>[2x]MNMTELKGALIGCGFFAVNQMHAWKDV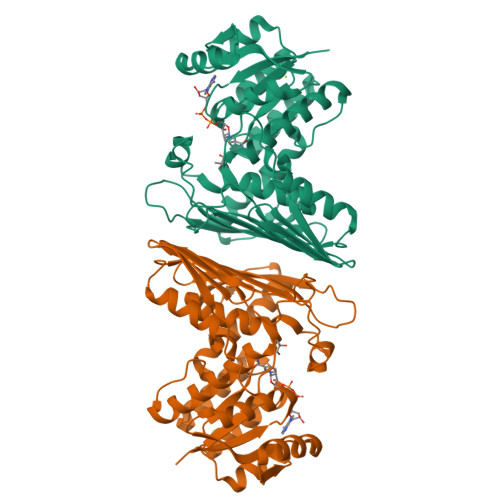KGAGIAAICDRDPKRLKLVGDQFGIERRYGDAAALFADGGFDFVDIATTVQSHRALVEMAAAHKVPAICQKPFAKSLSDAKAMVRTCENADIPLMVHENFRWQTPIQAVKAVLESGAIGEPFWGRFSFRSGFDVFSGQPYLAEGERFIIEDLGIHTLDIARFILGDVATLTARTKRVNPKIKGEDVATILLDHQNGATSIVDVSYATKLGTEPFPETLIDIDGTQGTIRLSQGYRLEVTGPNGMTISDASPQLLSWASRPWHNIQESVLAIQQHWTDRLSSGGETSTSGADNLKTFALVEAAYESAANGRTVDIGAML> MLLAALLAALVARTTLGADVDAVPAPTFPPPAYPYTESWQLTLTTVPSPFVGPADVYHTRPLEDPCGVVALISDPQVDRLLNEAVAHRRPTYRAHVAWYRIADGCAHLLYFIEYADCDPRQVFGRCRRRTTPMWWTPSADYMFPTEDELGLLMVAPGRFNEGQYRRLVSVDGVNILTDFMVALPEGQECPFARVDQHRTYKFGACWSDDSFKRGVDVMRFLT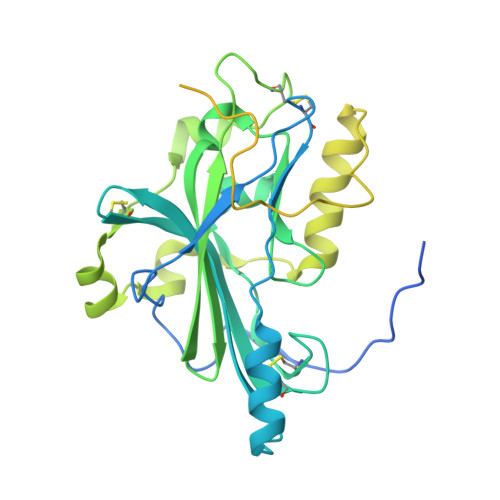PFYQQPPHREVVNYWYRKNGRTLPRAYAAATPYAIDPARPSAGSPRPRPRPRPRPRPKPEPAPATPAPPDRLPEPATRDHAAGGRPTPRPPRPETPHRPFAPPAVVPSGWPQPAEPFQPRTPAAPGVSRHRSVIVGTGTAMGALLVGVCVYIFFRLRGAKGYRLLGGPADADELKAQPGP>SPNYDKWEMERTDITMKHKLGGGQYGEVYEGVWKKYSLTVAVKTLKEDTMEVEEFLKEAAVMKEIKHPNLVQLLGVCTREPPFYIITEFMTYGNLLDYLRECNRQEVNAVVLLYMATQISSAMEYLEKKNFIHRDLAARNCLVGENHLVKVADFGLSRLMTGDTYTAHAGAKFPIKWTAPESLAYNKFSIKSDVWAFGVLLWEIATYGMSPYPGIDLSQVYELLEKDYRMERPEGCPEKVYELMRACWQWNPSDRPSFAEIHQAFET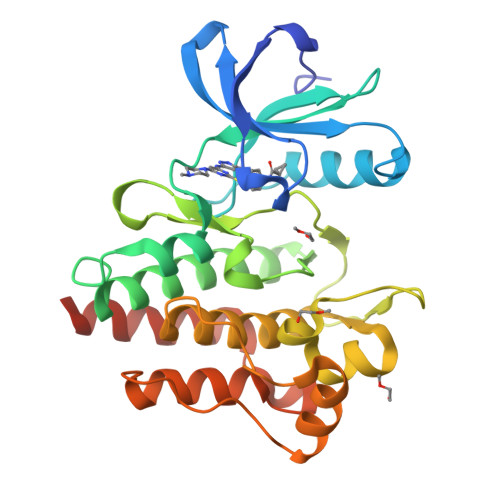MFQESSISDEVEKELG[2x]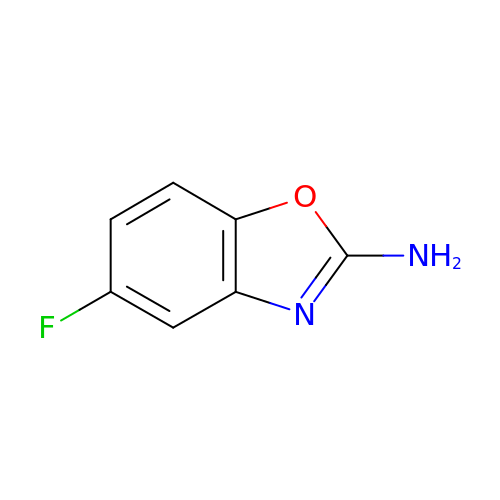5-fluoranyl-1,3-benzoxazol-2-amine | C7 H5 F N2 O | PFPSBRGOJCFWKD-UHFFFAOYSA-N>GPGSMRSLEDKNRTNTDDIRSLRVITAIKTPYLPDGRFDLQAYDDLVNTQIENGAEGVIVGGTTGEGQLMSWDEHIMLIGHTVNCFGGRIKVIGNTGSNSTREAIHATEQGFAMGMHGALHINPYYGKTSIEGMNAHFQTVLHMGPTIIYNVPGRTCQDIPPQVIFKLSQNPNMAGVKECVGNNRVEEYTEKGIVVWSGNDDQCHDSRWDHGATGVISVTSNLVPGLMRKLMFEGRNSALNAKLLPLMDWLFQEPNPIGVNTALAQLGVARPVFRL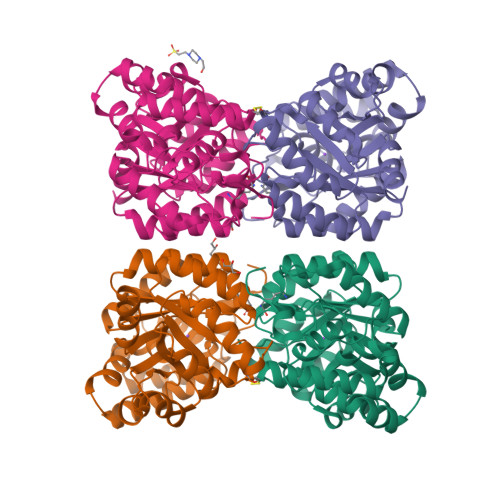PYVPLPLSKRIEFVKLVKEIGREHFVGDRDVQVLDDDDFILIGRY[4x]> MSFVDHPPDWLEEVGEGLREFLGLEAGPPKPKPNQQHQDQARGLVLPGYNYLGPGNGLDRGEPVNRADEVAREHDISYNEQLEAGDNPYLKYNHADAEFQEKLADDTSFGGNLGKAVFQAKKRVLEPFGLVEEGAKTAPTGKRIDDHFPKRKKARTEEDSKPSTSSDAEAGPSGSQQLQIPAQPASSLGADTMSAGGGGPLGDNNQGADGVGNASGDWHCDSTWMGDRVVTKSTRTWVLPSYNNHQYREIKSGSVDGSNANAYFGYSTPWGYFDFNRFHSHWSPRDWQR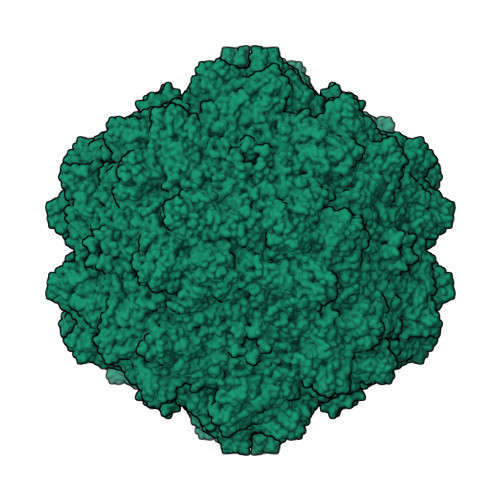LINNYWGFRPRSLRVKIFNIQVKEVTVQDSTTTIANNLTSTVQVFTDDDYQLPYVVGNGTEGCLPAFPPQVFTLPQYGYATLNRDNGDNPTERSSFFCLEYFPSKMLRTGNNFEFTYSFEEVPFHCSFAPSQNLFKLANPLVDQYLYRFVSTSATGAIQFQKNLAGRYANTYKNWFPGPMGRTQGWNTSSGSSTNRVSVNNFSVSNRMNLEGASYQVNPQPNGMTNTLQGSNRYALENTMIFNAQNATPGTTSVYPEDNLLLTSESETQPVNRVAYNTGGQMATNAQNATTAPTVGTYNLQEVLPGSVWMERDVYLQGPIWAKIPETGAHFHPSPAMGGFGLKHPPPMMLIKNTPVPGNITSFSDVPVSSFITQYSTGQVTVEMEWELKKENSKRWNPEIQYTNNYNDPQFVDFAPDGSGEYRTTRAIGTRYLTRPL>GHMAKTYDYLFKLLLIGDSGVGKTCVLFRFSEDAFNSTFISTIGIDFKIRTIELDGKRIKLQIWDTAGQERFRTITTAYYRGAMGIMLVYDITNEKSFDNIRNWIRNIEEHASADVEKMILGNKCDVNDKRQVSKERGEKLALDYGIKFMETSAKANINVENAFFTLARDIKAKMDKKLEGNSPQG[2x];>[4x]GPGYERLKEELAKAQRELKLKDEECERLSKVRDQLGQELEELTASLFEEAHKMVREANIK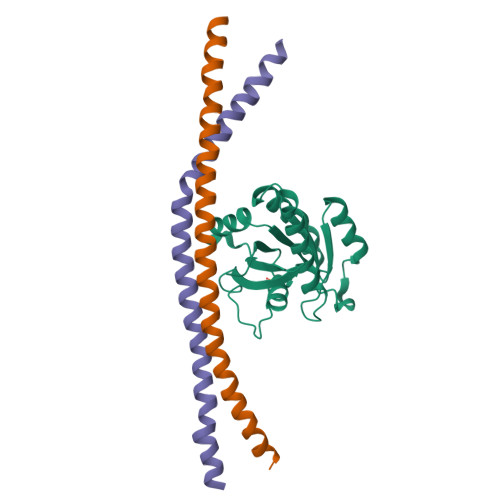QATAEKQLKEAQGKIDVL> MNSSKETKSEPSDSKKLMDQPYSKTDFLMGTVVTLKIYDKGKEDVLDKGFDRIKDLAAKITTSDSEKTSEVDKINEQAGKKPVKVSEDVYYLIQEGLKYSENSGGSFDITIGPLTSLWHI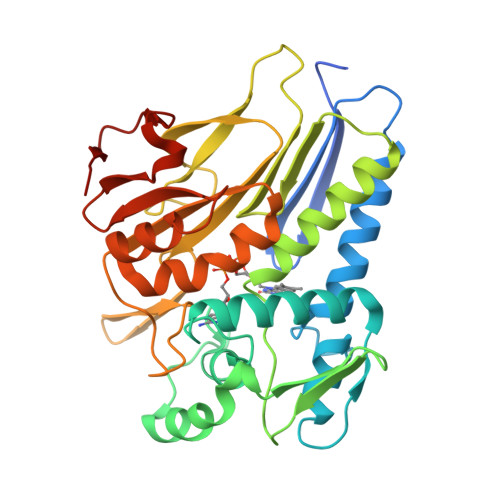GFSDARKPSQAEIDAVLPLINYKDVKMNDKDQTVYLEKEGMELDLGAIAKGFITDETLKVFKENKVTTSIIDLGGNIYVQGNNPNGNKWNVGIQDPFSPRGSVIGKLPESNMSIVTSGIYERYLEVDGKTYHHILDPKTGYPFDNDIAGVSIVSKKSIDGDGLSTATFSKGIKGGMDYIEQFEGVDAIFISKEKKVYETSGLKGQFELTDKDFQMDTLKK>[9x]MNRDHFYTLNIAEIAERIGNDDCAYQVL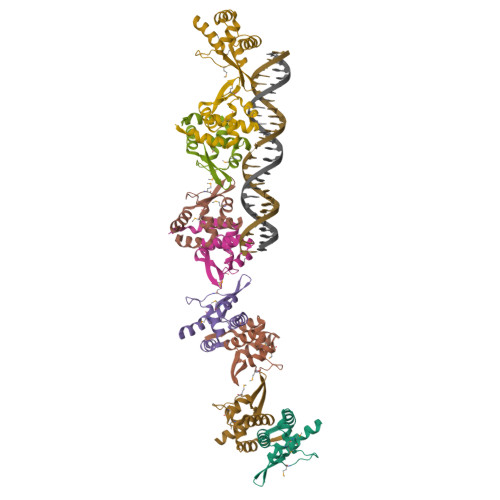MAFINENGEAQMLNKTAVAEMIQLSKPTVFATVNSFYCAGYIDETRVGRSKIYTLSDLGVEIVECFKQKAMEMRNL> MEEVVIAGMSGKLPESENLQEFWDNLIGGVDMVTDDDRRWKAGLYGLPRRSGKLKDLSRFDASFFGVHPKQAHTMDPQLRLLLEVTYEAIVDGGINPDSLRGTHTGVWVGVSGSETSEALSRDPETLVGYSMVGCQRAMMANRLSFFFDFRGPSIALDTACSSSLMALQNAYQAIHSGQCPAAIVGGINVLLKPNTSVQFLRLGMLSPEGTCKAFDTAGNGYCRSEGVVAVLLTKKSLARRVYATILNAGTNTDGFKEQGVTFPSGDIQEQLIRSLYQSAGVAPESFEYIEAHGTGTKVGDPQELNGITRALCATRQEPLLIGSTKSNMGHPEPASGLAALAKVLLSLEHGLWAPNLHFHSPNPEIPALLDGRLQVVDQPLPVRGGNVGINSFGFGGSNVHIILRPNTQPPP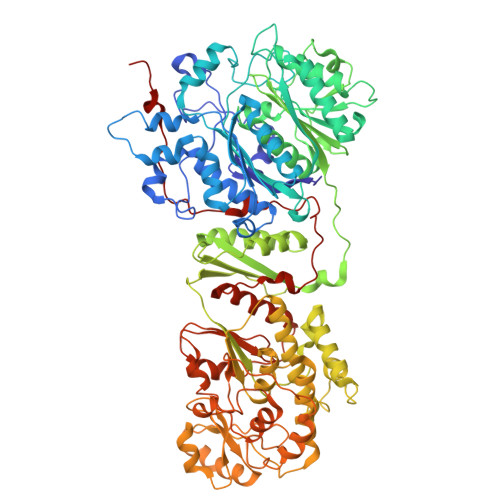APAPHATLPRLLRASGRTPEAVQKLLEQGLRHSQDLAFLSMLNDIAAVPATAMPFRGYAVLGGERGGPEVQQVPAGERPLWFICSGMGTQWRGMGLSLMRLDRFRDSILRSDEAVKPFGLKVSQLLLSTDESTFDDIVHSFVSLTAIQIGLIDLLSCMGLRPDGIVGHSLGEVACGYADGCLSQEEAVLAAYWRGQCIKEAHLPPGAMAAVGLSWEECKQRCPPGVVPACHNSKDTVTISGPQAPVFEFVEQLRKEGVFAKEVRTGGMAFHSYFMEAIAPPLLQELKKVIREPKPRSARWLSTSIPEAQWHSSLARTSSAEYNVNNLVSPVLFQEALWHVPEHAVVLEIAPHALLQAVLKRGLKPSCTIIPLMKKDHRDNLEFFLAGIGRLHLSGIDANPNALFPPVEFPAPRGTPLISPLIKWDHSLAWDVPAAEDFPNGS> NQPFAWQVASLSERYQEQFDIGAAVEPYQLEGRQAQILKHHYNSLVAENAMKPVSLQPREGEWNWEGADKIVEFARKHNMELRFHTLVWHSQVPEWFFIDENGNRMVDETDPEKRKANKQLLLERMENHIKTVVERYKDDVTSWDVVNEVIDDDGGLRESEWYQITGTDYIKVAFETARKYGGEEAKLYINDYNTEVPSKRDDLYNLVKDLLEQGVPIDGVGHQSHIQIGWPSIEDTRASFEKFTSLGLDNQVTELDMSLYGWPPTGAYTSYDDIPEELFQAQADRYDQLFELYEELSATISSVTFWGIADNHTWL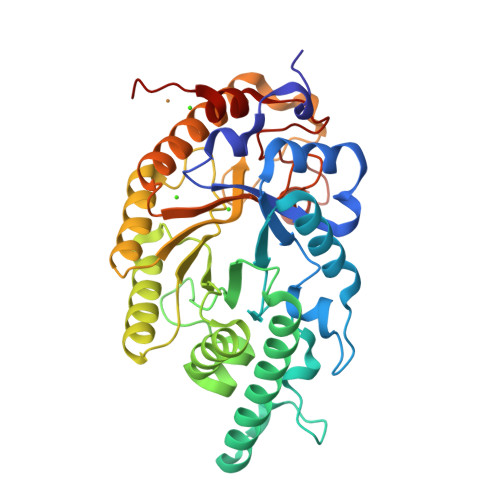DDRAREYNNGVGVDAPFVFDHNYRVKPAYWRIIDHHHHHH>GMETFKQQKVEDFYDIGEELGSGQFAIVKKCREKSTGLEYAAKFIKKRQSRASRRGVCREEIEREVSILRQVLHPNIITLHDVYENRTDVVLILELVSGGELFDFLAQKESLSEEEATSFIKQILDGVNYLHTKKIAHFDLKPENIMLLDKNIPIPHIKLIDFGLAHEIEDGVEFKNIFGT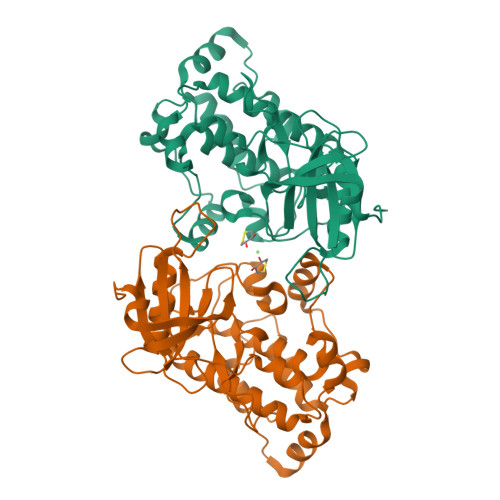PEFVAPEIVNYEPLGLEADMWSIGVITYILLSGASPFLGDTKQETLANITAVSYDFDEEFFSQTSELAKDFIRKLLVKETRKRLTIQEALRHPWITPVDTQQAMVRRESVVNLENFKKQYVRRRWKLSFSIVSLCNHLTRSLMKKVHLRTSEDLRNCESDTEENIARRKALHPRRRSSTS[2x]>GSFTMNLNFSLLDEPIPLRGGTILVLEDVCVFSKIVQYCYQYEEDSELKFFDHKMKTIKESEIMLVTDILGFDVNSSTILKLIHADLESQFNEKPEVKSMIDKLVATITELIVFECLENELDLEYDEITILELIKSLGVKVETQSDTIFEKCLEILQIFKYLTKKKLLIFVNSGAFLTKDEVASLQEYISLTNLTVLFLEPRELYDFPQYILDEDYFLITKNMV[2x]

Mounting evidence indicates that CRISPR and Cas proteins represent a microbial immune system that protects against invading foreign genetic elements, such as plasmids and phages. Csn2 is one of four Cas proteins that comprise the Nmeni subtype of the CRISPR/Cas system. The results of the mobility shift assay indicate that S. pyogenes Csn2 has a non-specific dsDNA-binding function. The tetrameric nature of S. pyogenes Csn2 results in a diamond-shaped ring structure with a positively charged inner surface as seen in E. faecalis Csn2.

The only CA2 site in the asymmetric unit of the S. pyogenes Csn2 structure is located adjacent to one of the two hinge regions in monomer A. The calcium ion in the CA2 site is coordinated by three residues (Glu138, Asp142, and Glu150) from monomer A, Asp118 from monomer B of the symmetry-related dimer, and two water molecules. In the corresponding hinge region of monomer B in the asymmetric unit, we were unable to locate a calcium ion. Based on these observations, we concluded that, indeed, no calcium ion was bound in the potential CA2 site adjacent to the hinge region of monomer B. This may indicate that the two types of calcium-binding sites, CA1 and CA2, have different affinities for calcium ions. The absence of calcium could also be a simple artifact caused by release of the calcium ion from the more exposed binding site during purification. It is important to note that the lack of a calcium ion is not a result of the selenomethionine (SeMet) labeling as our 2.9 Å native data also indicated the absence of calcium at this site. In contrast, we purified and crystallized S. pyogenes Csn2 without the addition of excess calcium ions.> NKIAHAMETKPRTPVIWLHGLECTCCSESFIRSAHPLAKDVVLSMISLDYDDTLMAASGHAAEAILDEIKEKYKGNYILAVEGNPPLNQDGMSCIIGGRPFSEQLKRMADDAKAIISWGSCASWGCVQAAKPNPTQATPVHKF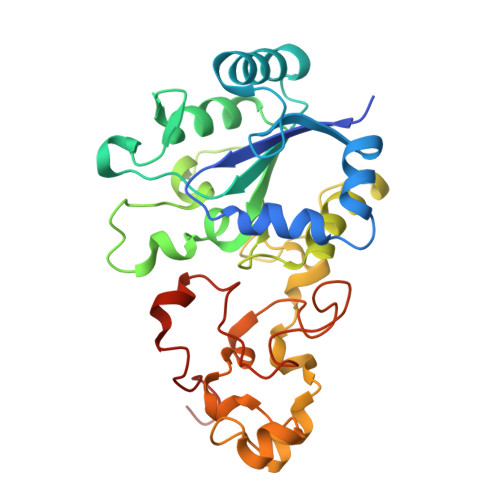LGGGYDKPIIKVPGCPPIAEVMTGVITYMLTFDRIPELDRQGRPKMFYSQRIHDKCYRRPHFDAGQFVEEWDDEGARKGYCLYKVGCKGPTTYNACSTVRWNGGTSFPIQSGHGCIGCSEDGFWDKGSFYSRDTEMNAFG> MSLIGEILPLSHIVLDMEVGSKKRLFEEAGLLLERESSLSHADVFECLFAREKLGSTGLGQGVAIPHGRHAGVKQATGAFIRTREPVGFDAPDGKPVSLIFILLVPENATGEHLEVLSKLAGKFSQKSIRESLMTVSSAEEVRAILTEE

The NMB0736 gene of Neisseria meningitidis serogroup B strain MC58 encodes the putative nitrogen regulatory protein, IIANtr (abbreviated to NM-IIANtr). IIANtr is a member of the mannitol-fructose family of IIA protein/domains which forms part of the phosphoenolpyruvate: sugar phosphotransferase system (PTS). PTS controls sugar uptake by bacteria through a series of phosphoryl transfer reactions in which the sugar-specific IIA enzyme is phosphorylated on a highly conserved histidine residue by the histidine-containing phosphocarrier protein, HPr. The sequence similarity between HPr and the molybdenum-iron protein of the nitrogenase complex of Rhizobium trifolii and the frequent association of PTS proteins with rpoN have been taken to suggest that IIANtr may provide a regulatory link between carbon and nitrogen assimilation in bacteria.

Analyses of re-dissolved crystals of the protein by mass spectrometry showed that only the un-phosphorylated form of the protein was crystallized presumably due to labile nature of the phospho-histidine bond in the acidic crystallisation conditions, 0.1 M sodium citrate, pH 4 (data not shown). The model of NM-IIANtr contains 146 (out of 149) protein residues and 72 water molecules. Residues 1 and 148–149 are not modelled in the structure due to lack of clearly defined electron density. The structure of NM-IIANtr consists of a 5-stranded mixed β-sheet which is sandwiched by six α-helices, two on one side and four on the other (Fig. 1a &1b). The overall fold, as expected from the sequence homology, is similar to that of E. coli IIANtr (34 % sequence identity) and IIAmtl (23% sequence identity). The major differences between the neisserial and E. coli structures appear at surface loops linking the secondary structure elements, for examples α2–α3, β3–β4 and β5-α4 loops (residues 34–40, 70–75 and 107–112 respectively in NM-IIANtr), and the termini. The active site of NM-IIANtr is located in a concave area of protein surface consisting of α3–α4 and β2–β3. The active site residue, H67, the equivalent of H73 in E. coli IIANtr or H65 in E. coli IIAmtl, is the fifth residue of β3 and is surrounded by hydrophobic residues L69, I65, L114, L117 and A121 on one side, and by hydrophilic residues R51 and R69 on the other side. The side-chain of R69 is folded toward the active site H67 unlike the corresponding K75 of E. coli IIANtr, which is folded away from the active site H73. Interestingly, in our structure there is also a strong peak of electron density located on the 2-fold crystallographic axis, which could be modelled as a sulphate ion interacting with the side-chains of R51, H67 and R69 via salt bridge/hydrogen bonding, as well as to the equivalent residues of the symmetry related molecule.>[2x]HFLCGVVEGFYGRPWVMEQRKELFRRLQKWELNTYLYAPKDDYKHRMFWREMYSVEEAEQLMTLISAAREYEIEFIYAISPGLDITFSNPKEVSTLKRKLDQVSQFGCRSFALLFDNIDHNMCAADKEVFSSFAHAQVSITNEIYQYLGEPETFLFCPTEYCGTFCYPNVSQSPYLRTVGEKLLPGIEVLWTGPKVVSKEIPVESIEEVSKIIKRAPVIWDNIHANDYDQKRLFLGPYKGRSTELIPRLKGVLTNPNCEFEANYVAIHTLATWYKSNMNGVRKDVVMTDSEDSTVSIQIKLENEGSDEDIETDVLYSPQMALKLALTEWLQEFGVPHQYSSRGGGGSGGGGSVTLEDLQLLADLFYLPYEHGPKGAQMLREFQWLRANSSVVSVNCKGKDSEKIEEWRSRAAKFEEMCGLVMGMFTRLSNCANRTILYDMYSYVWDIKSIMSMVKSFVQWLGCRSHSSAQFLIGDQEPWAFRGGLAGEFQRLLPIDGANDLFFQ;>FPTSTSLSPFYLR[2x]

OGA is the unique enzyme responsible for O-GlcNAc hydrolysis from a large number of cytoplasmic and nuclear proteins. Recently, our group and others have independently identified crystallizable constructs of OGA that comprise the catalytic domain and stalk domain, and published the apo form structures and enzyme complexes with active site inhibitors. These reports consistently showed that OGA formed an unusual arm-in-arm homodimer, where the catalytic domain of one monomer covered by the stalk domain of the sister monomer to create a potential substrate-binding cleft. Exploiting our previously reported construct of OGAcryst (residues 60–704 with the unstructured insert residues 401–552 replaced by a glycine–serine (GS) linker), we solved the structures of a mutant OGAcryst-D175N (catalytically impaired but retaining the ability to bind substrate) in apo form and in complex with each of four synthetic glycopeptides.

In the substrate complexes, all the glycopeptides were bound in the OGA substrate-binding cleft. Particularly, the GlcNAc moieties were anchored by the same set of OGA residues in the catalytic pocket, displaying nearly identical binding conformations regardless of the glycosylated residues or the flanking peptide sequences. Consistent with the O-GlcNAc hydrolysis mechanism, the catalytic residue D174 was optimally positioned to make a hydrogen bond with the N-acetyl group of GlcNAc in all the complexed structures. The N175 mutant side chain played an important role in anchoring the glycosylated hydroxyl of serine or threonine and stabilizing the OGA substrate complexes. In addition to these common features, peptide specific interactions have also been detected. As an example, the α-crystallin B chain was stabilized in a V shape by a pair of hydrogen bonds between the peptide backbone and the N175 residue. The hydroxyl groups of threonine (+ 1 subsite) and serine (+ 2 subsite) were further stabilized by intra-molecular hydrogen bonds, while the aliphatic side chain of leucine (+ 3 subsite) made favorable van der Waals contacts with L141 on the inner surface of the substrate-binding cleft. We find that OGA is able to bind peptide substrates in different directions, but in a conserved conformation regardless of the glycosylation site or flanking sequences.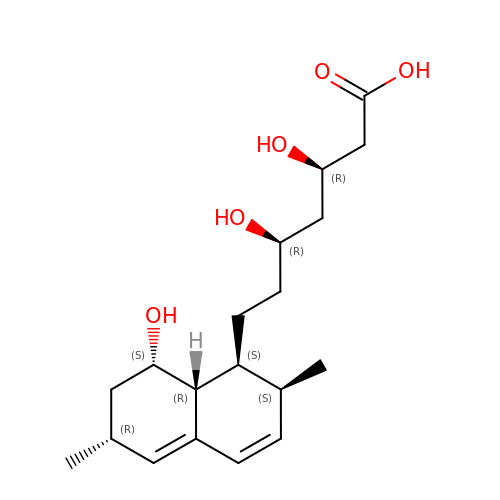(3R,5R)-3,5-dihydroxy-7-[(1S,2S,6R,8S,8aR)-8-hydroxy-2,6-dimethyl-1,2,6,7,8,8a-hexahydronaphthalen-1-yl]heptanoic acid | C19 H30 O5 | FJQFRDAWQRBFCG-IRUSZSJRSA-N>[4x]STLEIAGLVRKNLVQFGVGEKNGSVRWVMNALGVKD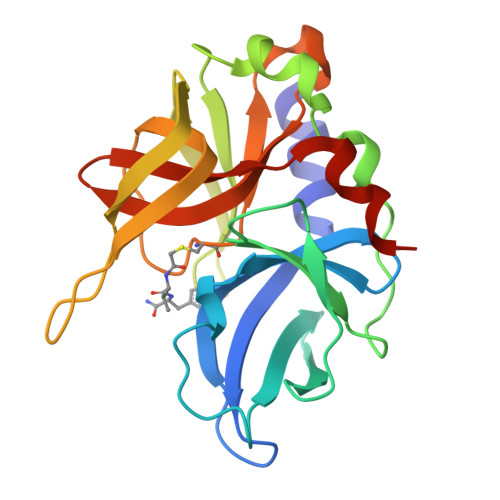DWLLVPSHAYKFEKDYEMMEFYFNRGGTYYSISAGNVVIQSLDVGAQDVVLMKVPTIPKFRDITQHFIKKGDVPRALNRLATLVTTVNGTPMLISEGPLKMEEKATYVHKKNDGTTVDLTVDQAWRGKGEGLPGMCGGALVSSNQSIQNAILGIHVAGGNSILVAKLVTQEMFQNIDKKIE> MATIAGLRGTGDWGNQERPTDFRETILWMEPNGQAPLQALMSKMSSQPTTDPEFSWWEEKLTHNRLEVKTEAAAGVTTLAVDTDQAWACVKGDILMVESVGGLWANEILKVVEDPTAGNALKV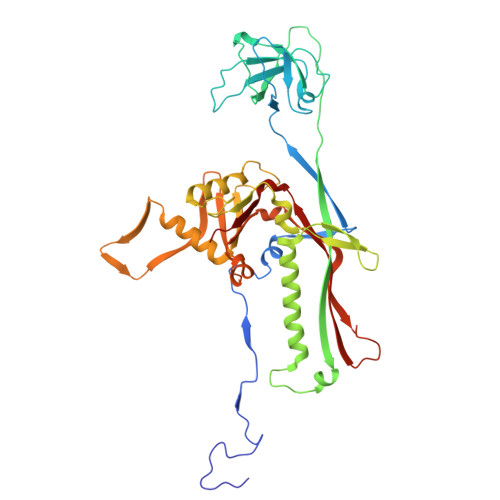ARGFAGTTAAVIPAGTFIIAIGTSFAEGSLAPKSATRNPVKLNNFCQIFKKSYEITKTADATKARTGSALANDKKRRMFDYYRDVEMAFIYGRKSETVGENGKPERTTGGLLNFITTNRTQFGTGAGKTELTEDSLIDFFANVFNYDGQGAGNQRIAFVGNTALTKINKLARNSPSTRINFDKQVTQVYGMNFTRWVLPQGEIFFKTHPLFNVHPELSKAMMVLNPKGIKERVLRATKPENDIQQVGQDSIKGQWIGEFGLEVNHEETMAFAGGIA> G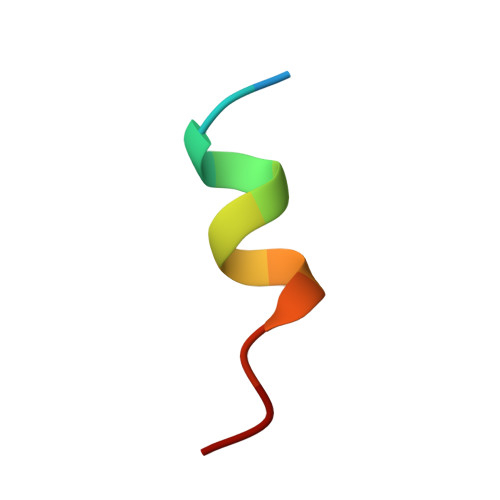HKILHRLLQDSS2-[2,4-bis(oxidanyl)phenyl]-3,5,7-tris(oxidanyl)chromen-4-one | C15 H10 O7 | 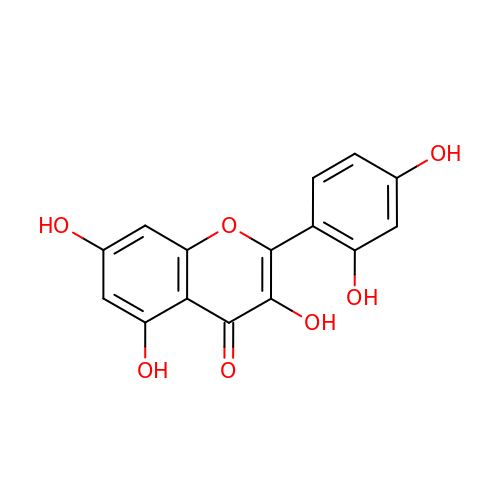YXOLAZRVSSWPPT-UHFFFAOYSA-N> MNGIHDVGGMDGFGKVMYVKEEEDIYFTHDWERLAFGLVAGCMAQGLGM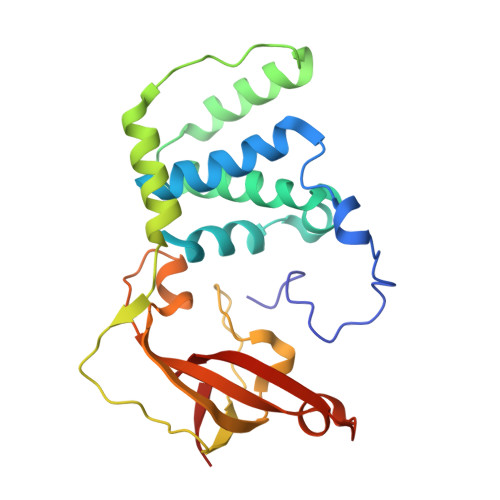KAFDEFRIGIELMRPVDYLTSSYYGHWIATVAYNLVDTGVLDEKELDERTEVFLKKPDTKIPRREDPALVKLVEKALYDGLSPLREISASPRFKVGERIKTKNIHPTGHTRFPRYARDKYGVIDEVYGAHVFPDDAAHRKGENPQYLYRVRFEAEELWGYKQKDSVYIDLWESYMEPVSH> IVGGYTCGANTVPYQVSLNSGYHFCGGSLINSQWVVSAAHCYKSGIQVRLGEDNINVVEGNEQFISASKSIVHPSYNSETYNNDIMLIKLKSAASLNSRVASISLPTSCASAGTQCLISGWGNTKSSGTSYPDVLKCLKAPILSDSSCKSASSFIITSNMFCAGYLEGGKDACQGDSGGPVVCSGKL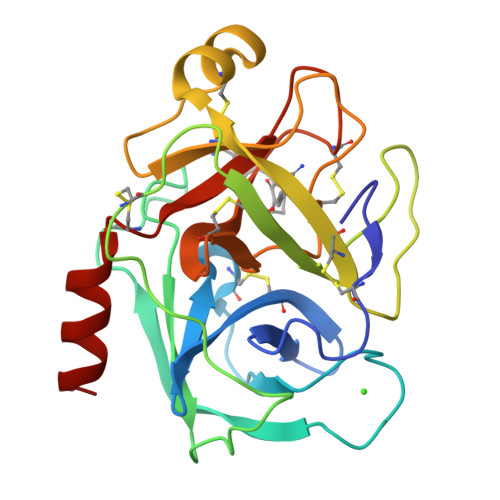QGIVSWGSGCAQKNKPGVYTKVCNYVSWIKQTIASN>MSLKIRDAYTIVTCPGRNFVTLKIVTESGTHGIGDATLNGREMAVAAYLDEHVVPALIGRDAGRIEDTWQYLYRGAYWRRGPVTMTAIAAVDMALWDIKAKAAGMPLYQLLGGKSRERVMTYAHCTGQTIEDCLGEVARHVELGYRAVRVQSGVPGIETTYGVAKTPGERYEPADSSLPAEHVWSTEKYLNHAPKLFAAVRERFGD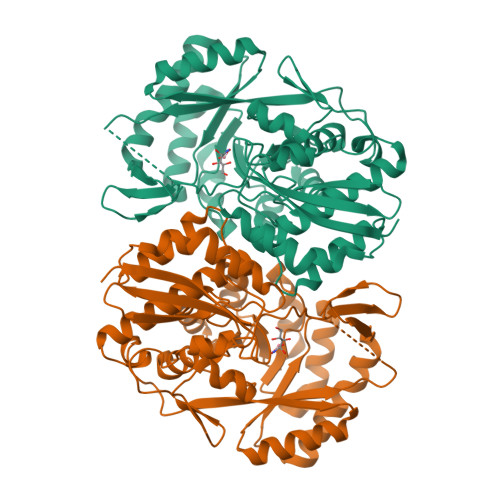DLHVLHDVHHRLTPIEAARLGKAVEPYHLFWLEDCVPAENQESLRLIREHTTTPLAIGEVFNSIHDCRELIQNQWIDYIRMPLTHGGGITAMRRVADLASLYHVRTGFHGPTDLSPVCLGAAIHFDTWVPNFGIQEHMPHTDETDAVFPHDYRFEDGHFLAGESPGHGVDIDEELAAKYPYERASLPVNRLEDGTLWHW[4x]>[2x]GMEDLIPLVNRLQDAFSAIGQNADLDLPQIAVVGGQSAGKSSVLENFVGRDFLPRGSGIVTRRPLVLQLVNATTEYAEFLHCKGKKFTDFEEVRLEIEAETDRVTGTNKGISPVPINLRVYSPHVLNLTLVDLPGMTKVPVGDQPPDIEFQIRDMLMQFVTK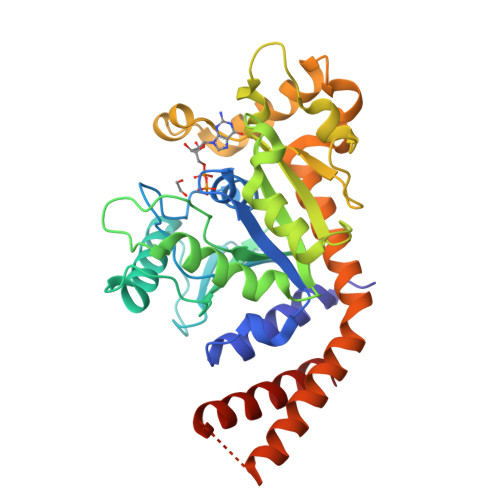ENCLILAVSPANSDLANSDALKVAKEVDPQGQRTIGVITKLDLMDEGTDARDVLENKLLPLRRGYIGVVNRSQKDIDGKKDITAALAAERKFFLSHPSYRHLADRMGTPYLQKVLNQQLTNHIRDTLPGLRNKLQSQLLSIEKEVEEYKNFRPDKHGTDSRVDEMLRMYHALKEALSIIGDIN> SMSKKQEYIAPIKYQNSLP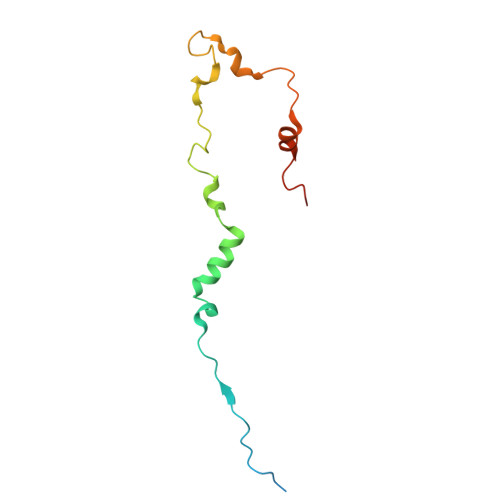VPQLPPKLLAYPEAPETNPDSSQLINSLYVKTNISNLIQQDEDLGMPVDLMKFPGLLNKLDSKLLYGFDNVKLDKDDRILLRDPRIDRLTKT>MVLDVTKDHWLPYVLLAQLPVMVLFRKDNDEEAKKVEYIVRELAQEFDGLIRVFYVDINKAPEIAKKYNITTTPTVAFFHNGELKSVFTGAITKDQLRDEILKYLGLEHHHHHH[2x]

As a proof of concept, we enhanced the stability of a marginally stable designed protein (called dF106) through conventional directed evolution. dF106 was created in an effort to computationally redesign the ubiquitous Rossmann fold of thioredoxins using Rosetta Design. Using the CPOP system, dF106 variants were selected, genetically resulting in a protein variant dF106-L11P-D83V, henceforth termed enhanced dF106 (edF106). This had a high stability with a folding energy of −48 kJ/mol. Crystal structures of stabilized variants showed small perturbations in helices 1 and 2, which rendered them closer in structure to the redesign template.

We therefore introduced the 15 substitutions predicted to be most stabilizing by the GMMA into the isolated edF106 protein to measure their individual as well as combined effects on thermodynamic stability. The top 15 substitutions are found at nine distinct positions, with some positions having two or three substitutions that GMMA suggests are stabilizing. Thus, only nine could be combined to form the multi-mutant 9 (MM9) variant. All the same, the MM9 variant had a stability of −68.6 ± 1.1 kJ/mol (ΔΔG = −21.8 ± 1.1 kJ/mol, n = 5) and an extrapolated melting temperature of 152°C ± 10°C (n = 5). To gain more insight into the effects of the mutations, we crystalized and determined the crystal structure of MM9 using diffraction data that extended to a resolution at 1.9 Å. However, there was no visible electron density to fit the N-proximal residues (1–17). Instead, a strong crystal contact was present on the exposed surface and had likely moved the 17-residue helix (α1) out of the way. The crystals grew very slowly, typically within a month, with a low success rate out of 48 examined crystallization conditions. Only one or two would yield crystals indicative of a conformational change taking place in order to stabilize the crystal lattice. The structure also revealed that the destabilizing substitution E54Y presented in MM9, but not in eMM9, would probably be incompatible with the native conformation of Val2, which may have facilitated its increased dynamics following MM9 crystal formation.>[4x]MSLIKNPILRGFNPDPSICRAD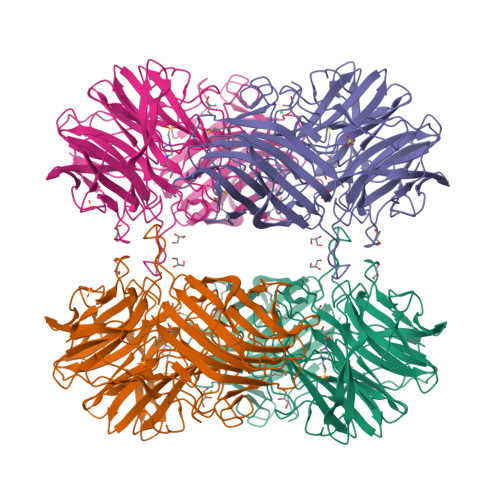TDYYIATSTFEWFPGVQIHHSKDLVNWHLVAHPLNRTSLLDMKGNPNSGGIWAPDLSYHDGKFWLIYTDVKVTDGMWKDCHNYLTTCESVDGVWSDPITLNGSGFDASLFHDNDGKKYLVNMYWDQRTYNHNFYGIVLQEYSDKEKKLIGKAKIIYKGTDIKYTEGPHIYHIGDYYYLFTAEGGTTYEHSETVARSKNIDGPYEIDPEYPLLTSWHDPRNSLQKCGHASLVHTHTDEWYLAHLVGRPLPVGNQPVLEQRGYCPLGRETSIQRIEWVDNWPRVVGGKQGSVNVEAPKIPEVKWEKTYDEKDNFDSDKLNINFQSLRIPLTENIASLKAKKGNLRLYGKESLTSTFTQAFIARRWQSFKFDASTSVSFSPDTFQQAAGLTCYYNTENWSTIQVTWNEDKGRVIDIVCCDNFHFDMPLKSNVIPIPKDVEYIHLKVEVRVETYQYSYSFDGINWSKVPAIFESRKLSDDYVQGGGFFTGAFVGINCIDITGNNKPADFDYFCYKEEGHHHHHH>MKAVLEQFGFPLTGTEARCYTNHALSYDQAKRVPRWVLEHISKSKIMGDADRKHCKFKPDPNIPPTFSAFNEDYVG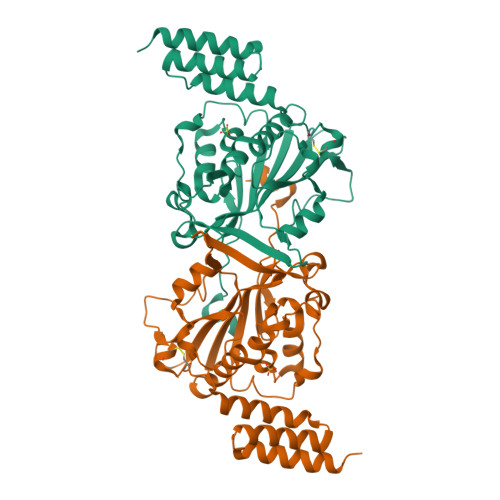SGWSRGHMAPAGNNKFSSKAMAETFYLSNIVPQDFDNNSGYWNRIEMYCRELTERFEDVWVVSGPLTLPQTRGDGKKIVSYQVIGEDNVAVPSHLYKVILARRSSVSTEPLALGAFVVPNEAIGFQPQLTEFQVSLQDLEKLSGLVFFPHLDRTSDIRNICSVDTCKLLDFQEFTLYLSTRKIEGARSVLRLEKIMENLKNAEIEPDDYFMSRYEKKLEELKAKEQSGTQIRKPSHHHHHH[2x]> MLARYLDPSVHPLRVGQVVAYDYLHAAKTWQWTLGTVREIKDYTAVVQQWGLHTGDIDTLRSILLKEVDTENGRMKNYHDMLAIAREKLASIRRSNEDRVSHVRGHFDKAREKVELIDEVDLRKVTAQAAPSPVAVAVLKAVWAVAKCDPTAVEFYEWADVQLEYRKPAALDEIAKTDVLAKLYPSAESLQQSLEQDPKLNYKAAARDSPVVASLHAWVITALAYQQAYNLLAHDKRIQEQNDAIAAAIAGMKACRAKIAKLKDELSSKDTAALPGQVTS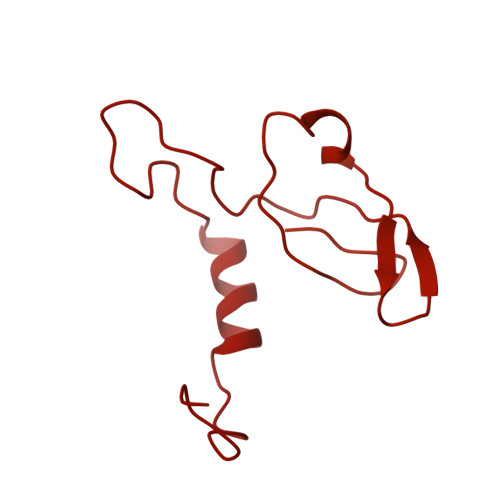FTRTSVLVTIPLSAVISPVNVDTDVKRCVLTKDEVEQIPIDAKITRYAQKQKLAITGSHLLDQYAAATTTHIYVTELEDRLFFFQHYMASALRDAQTAAVDAHQRLAVSLHELEAFRQKRHDAKKARAAEPELADADGVEPSSGPTSSRSPTGRAAPRGQSAAPRGTASQQHKLLGPAYQSIDPATIANEPLYAVTIEEYKAKDAAGERAMDEAERMADEVQRLAVELEDAKAAADKLAEELAAKDEELAAHRQKRHDAQQARASDPALAAADAVAPRSGKGAASPHVGAVQRQAVDPATVPVAPAVIAEEPLYVATAEELQHVRDFADQLAEELEAFRQKRHDAKKARAAEPELADADGVEPSSGPTSSRSPTGRAAPRGQSAAPRGTASQQHKLLGPAYQSIDPATIANEPLYAVTIEEYKAKDAAGERAMDEAERMADEVQRLAVELEDAKAAADKLAEELAAKDEELAAHRQKRHDAQQARASDPALAAADAVAPRSGKGAASPHVGAVQRQAVDPATVPVAPAVIAEEPLYVATAEELQHVRDFADQLAEELEAFRQKRHDAKKARAAEPELADADGVEPSSGPTSSRSPTGRAAPRGQSAAPRGTASQQHKLLGPAYQSIDPATIANEPLYAVTIEEYKAKDAAGERAMDEAERMADEVQRLAVELEDAKAAADKLAEELAAKDEELAAHRQKRHDAQQARASDPALAAADAVAPRSGKGAASPHVGAVQRQAVDPATVPVAPAVIAEEPLYVATAEELQHVRDFADQAAHDAATREAEVAGTVENLRNELDDVREMNAKLEDEVFALKEQLSDAEDAYKKLAGALVVAEDERQELCDDLEAALDELEQKKDEYDELLGNLEEVQGLLEAADVAGRTAVEALEQRNRDMADLQGELANALDASKENENLRALLDAKEREIDRLKEYNSFWTDTVGTGKQKVTHRLTKIFDGDWTRLMRHRPEALKAAFVIDSSNACHVPGDQIFLVSNSFTRRLLTRTDHCPKCDRLSTFRFMSVSGMVGRMPYKPVDTPGPSYATLYWRKQRSGKIASQPLNEVCNKNEF> HIIENPQYFSDACVHHIKRRDIVLKWELGEGAFGKVFLAECHNLLPEQDKMLVAVKALKEASESARQDFQREAELLTMLQHQHIVRF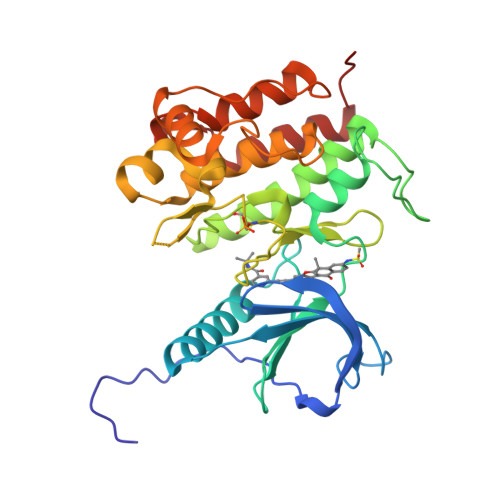FGVCTEGRPLLMVFEYMRHGDLNRFLRSHGPDAKLLAGGEDVAPGPLGLGQLLAVASQVAAGMVYLAGLHFVHRDLATRNCLVGQGLVVKIGDFGMSRDIYSTDYYRVGGRTMLPIRWMPPESILYRKFTTESDVWSFGVVLWEIFTYGKQPWYQLSNTEAIDCITQGRELERPRACPPEVYAIMRGCWQREPQQRHSIKDVHARLQALAQAPPVYL>[6x]M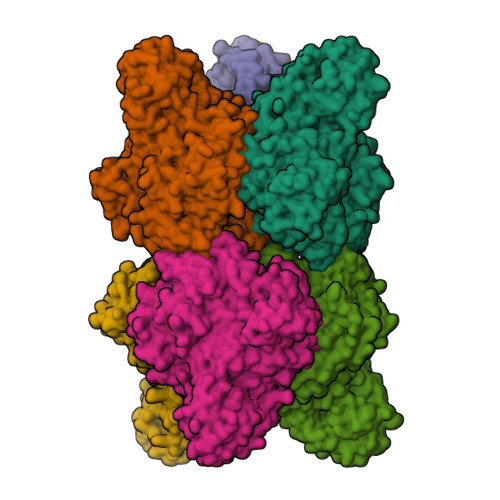RILKIYENKGVYKVVIGEPFPPIEFPLEQKISSNKSLSELGLTIVQQGNKVIVEKSLDLKEHIIGLGEKAFELDRKRKRYVMYNVDAGAYKKYQDPLYVSIPLFISVKDGVATGYFFNSASKVIFDVGLEEYDKVIVTIPEDSVEFYVIEGPRIEDVLEKYTELTGKPFLPPMWAFGYMISRYSYYPQDKVVELVDIMQKEGFRVAGVFLDIHYMDSYKLFTWHPYRFPEPKKLIDELHKRNVKLITIVDHGIRVDQNYSPFLSGMGKFCEIESGELFVGKMWPGTTVYPDFFREDTREWWAGLISEWLSQGVDGIWLDMNEPTDFSRAIEIRDVLSSLPVQFRDDRLVTTFPDNVVHYLRGKRVKHEKVRNAYPLYEAMATFKGFRTSHRNEIFILSRAGYAGIQRYAFIWTGDNTPSWDDLKLQLQLVLGLSISGVPFVGCDIGGFQGRNFAEIDNSMDLLVKYYALALFFPFYRSHKATDGIDTEPVFLPDYYKEKVKEIVELRYKFLPYIYSLALEASEKGHPVIRPLFYEFQDDDDMYRIEDEYMVGKYLLYAPIVSKEESRLVTLPRGKWYNYWNGEIINGKSVVKSTHELPIYLREGSIIPLEGDELIVYGETSFKRYDNAEITSSSNEIKFSREIYVSKLTITSEKPVSKIIVDDSKEIQVEKTMQNTYVAKINQKIRGKINLE>MGHHHHHHMAGEVVKSQKKRIRLGKVVPSSIRIVLDCAFDDLMNDKEINSLCQQVTRCHSANRTALHPVELFATNFGGRLKTRQDFVLKGQQNNWKRYNPTTKSYLEEFESQKEKLVYLSADSDNTITELDEDKIYIIGAIVDKNRYKNLCQNKASEQGIKTAKLPIDEYIKITDRKILTVNQVFEILSLWLEYRDWEKAFM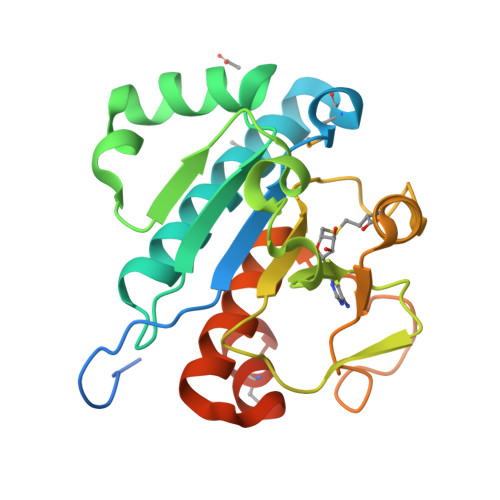EVIPKRKGILLKSDE[2x]> DLQLLHQKVEEQAAKY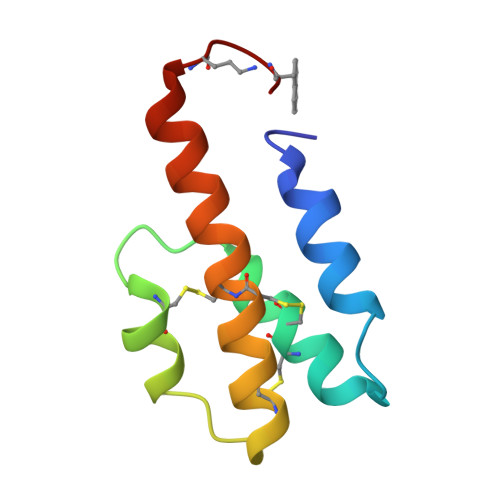KHRVPKKCCYDGARENKYETCEQRVARVTIGPHCIRAFNECCTIADKIRKNISHKFAPAAR>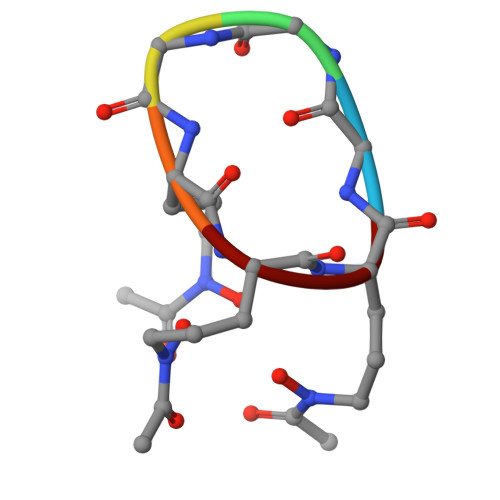 GGGAAA>[2x]GESWQKRYDSLQKIVEKQQQKMDQLRSQVQSLEQEVAQEEGTSQALREEAQRRDSALQQLRTAVKELSVQNQDLIEKNLTLQEHLRQA

Here we demonstrate that CEP85 is essential for faithful centriole duplication through a direct interaction with the previously uncharacterised N-terminal domain of STIL, a key factor involved in the early steps of centriole formation. Subsequently, through its C-terminal PB3, PLK4 interacts with STIL and phosphorylates it, enabling STIL to recruit SASS6 to the site of procentriole assembly.

Additional sidechain–sidechain hydrogen bonds and salt bridges act to further stabilize the dimer interface. As with the STIL NTD, we calculated the sequence conservation of the CEP85 coiled-coil (cc4) and mapped it onto its structure. This analysis showed the presence of a striking conservation on the outside of the coiled-coil towards its C-terminal end (within the dashed box) suggesting that this region might be involved in mediating protein–protein interactions. NMR and native, as well as cross-linking mass-spectrometry data support the notion of a direct interaction between the STIL NTD and the CEP85 cc4 domain. Further biophysical characterisations of the individual proteins in solution suggest that the STIL NTD is monomeric, while the CEP85 cc4 is in a monomer-dimer equilibrium at room temperature and at the concentrations and buffer conditions used in these biophysical studies while becoming predominantly dimeric at reduced temperatures. While we extend the spectrum of CEP85 activities by showing that its fourth coiled-coil domain interacts with STIL and thereby also plays a role in centriole duplication, the complexities of CEP85’s architecture suggest that it might have additional functions in vivo.>MPILQVQVTAGRSQQQKTAFLQNATKVIEQTLNAALPSIRISLHEIEQQDSIVAGQVGAEFVNIVAF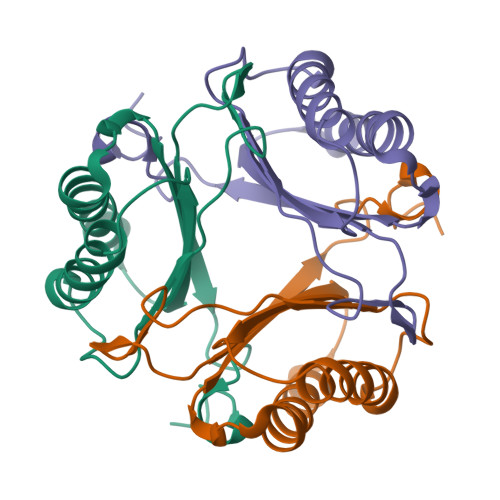LLAGRNDEVKANFLAAINKTAVTTLDVSDSCIRTMLIDIAPEHMGVQEGLSAAAFRARSAG[8x]> AAAAAA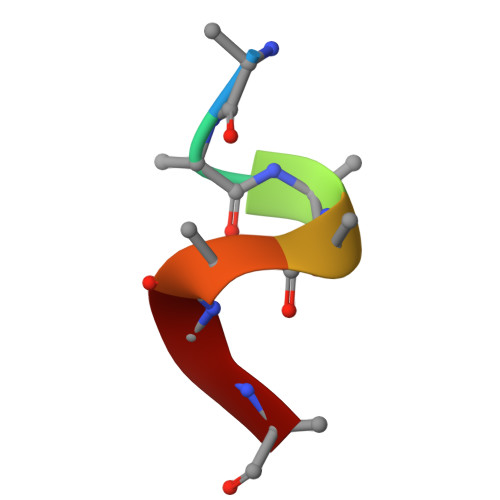A> GUUCCCGAAAGGAUGGCGGAAACGCCAGAUGCCUUGUAACCGAAAGG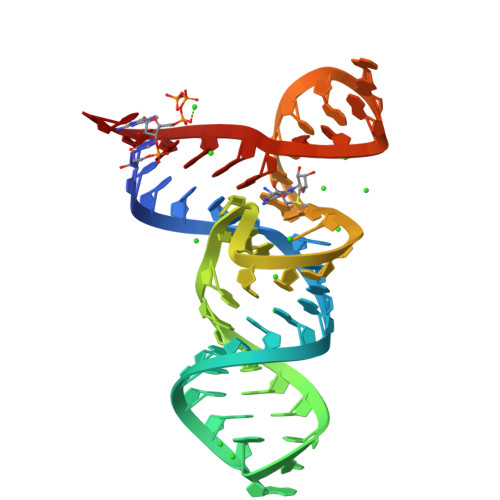GGGAAU(2R)-2-(4-oxoquinazolin-3(4H)-yl)propanoic acid | C11 H10 N2 O3 | 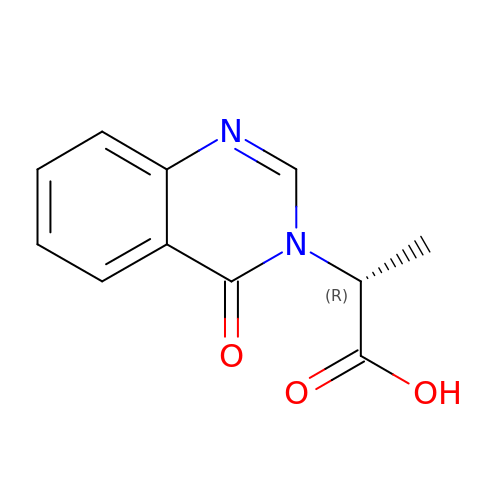AOIOGRLXASIYJK-SSDOTTSWSA-N>[2x]SHKEFTKFCYEVYNEIKISDKEFKEKRAALDTLRLCLKRISPDAELVAFGSLESGLALKNSDMDLCVLMDSRVQSDTIALQFYEELIAEGFEGAFLQAARIPIIKLTSDTKNGFGASFQCDIGFNNRLAIHNTLLLSSYTKLDARLKPMVLLVKHWAKRKQINSPYFGTLSSYGYVLMVLYYLIHVIKPPVFPNLLLSPLKQEKIVDGFDVGFDDKLEDIPPSQNYSSLGSLLHGFFAFYAYAFEPREKVVTFRRPDGYLTKQEKGWTSATEHTGSADQIIKDRYILAIEDPFEISHNVGRTVSSSGLYRIRGEFMAASRLLNSRSYPIPYDSLFEEAPIPPRRQKKTDEQSNKKLLNETDGDNSE

One such TUT family member, Cid1 from Schizosaccharomyces pombe, is a now well-characterized TUT, which was first demonstrated to be localized to the cytoplasm and to possess poly(A) polymerase activity in vitro, but more recently has been shown to possess TUT or poly(U) polymerase activity, in vitro and in vivo. The TUTactivity of Cid1 has been shown to be important in promoting mRNA degradation of polyadenylated and 3′ trimmed transcripts mediated by Lsm1–7 and the exonuclease Dis3l2 (12,13). Cid1 has been extensively characterized both structurally and biochemically, revealing that a single histidine (H336) in the nucleotide recognition motif (NRM) is predominantly responsible for discriminating uracil over other bases via a mechanism that was proposed to involve two alternative conformations of the H336 side chain. We used an RNA-binding-defective mutant of Cid1 (K133A/R137A/R277A/K282A) to improve the resolution of our crystal diffraction for higher resolution studies.

We have successfully improved the resolution of diffraction of our crystals, resulting in a higher resolution (1.74 Å) crystal structure of Cid1. The structure determined to 1.74 Å contains two molecules in the asymmetric unit with one chain exhibiting a typical Apo conformation and the other having a significantly different conformation. In one of the molecules in the asymmetric unit of our high resolution structure (chain A), presented here, we observe that indeed H336 adopts two conformations via a 180° rotation about the χ2 bond. Unexpectedly, this H336 flipping occurs as a result of a double conformation of the D330 side chain, which was clearly visible in the unbiased electron density. Therefore, the H336 flipping previously reported, which was inferred by analysis of the refined structure, has now been observed directly and can be explained by the hydrogen bonding network with D330 and several water molecules. Of the two molecules in the asymmetric unit of the high resolution crystal structure described in this paper, it was clear from the excellent quality unbiased electron density that the NTD of chain B had adopted an unusual conformation. This conformation is related to one seen in our previous report but the mutant enzyme used for this study is trapped in an intermediate stage compared to the previous closed form. Dyndom analysis indicates a pivot point for the domain motion of this ‘intermediate’ structure as residues 163–172, supporting the idea that there is an inherent flexibility within the enzyme between the two domains and that there is a single hinge point about which it occurs. We analysed the volume of the catalytic cleft of Cid1 and its intermediate closed conformer using 3V, and found that in a native open conformation the catalytic cleft volume accessible by solvent is 3339Å3 whereas the NTD rotation reduces the volume of the catalytic cleft by approximately a factor of 10 (336 Å3).>[2x]SNAMTSLEEITKAIMADSQNKVFTEKNIEPLFAAPKTARINIVGQAPGIKAQESRLYW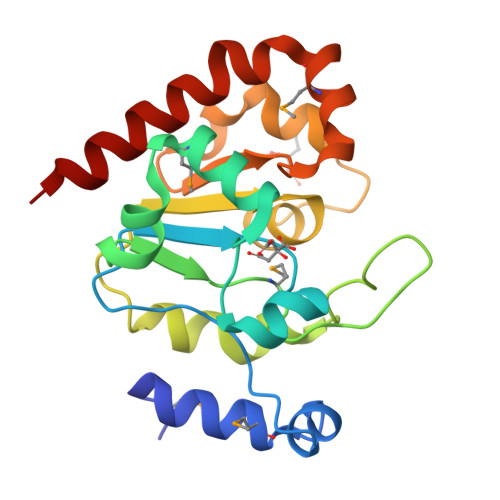NDKSGDRLREWMGVDYDTFYHSGYFAVIPMDFYYPGKGKSGDLPPRKGFAQKWHQPILDLLPDIQLTILIGNYAQKYYLHQKSSVKLTDTVAHYKKYLPDYFPLVHPSPRNQIWMSRHPWFEAQVVPDLKKIIQQIIQSS>ALLQKTRIINSMLQAAAGKPVNFKEMAETLRDVIDSNIFVVSRRGKLLGYSINQQIENDRMKKMLEDRQFPEEYTKNLFNVPETSSNLDINSEYTAFPVENRDLFQAGLTTIVPIIGGGERLGTLILSRLQDQFNDDDLILAEYGATVVGMEILREKAEEIE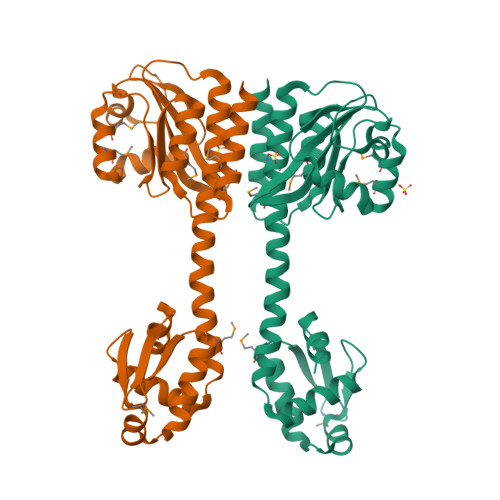EEARSKAVVQMAISSLSYSELEAIEHIFEELDGNEGLLVASKIADRVGITRSVIVNALRKLESAGVIESRSLGMKGTYIKVLNNKFLIELENLKSHHHHHH[10x]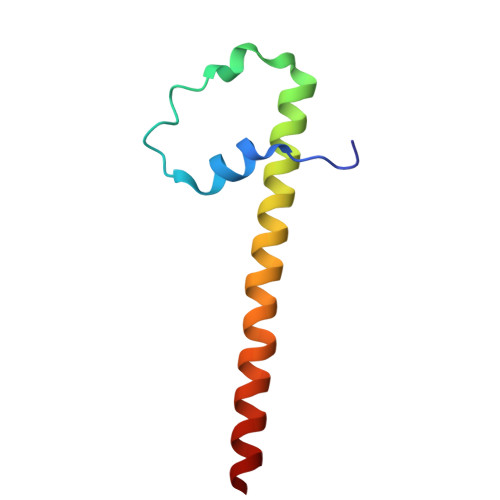> LLEEIPKWLAVYSEADSSKDHLLQFNMFSLPELEGFDSMLVRLFKQELGTIVGFYERYRRALILEKNRRA>[2x]MAKLTSAVPVLTARDVAEAVEFWTDRLGFSRV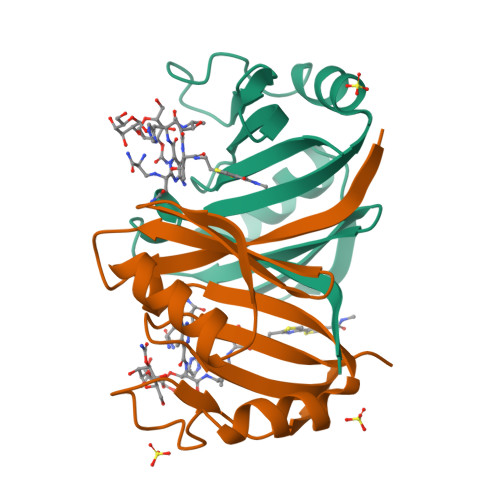FVEDDFAGVVRDDVTLFISAVQDQVVPDNTQAWVWVRGLDELYAEWSEVVSTNFRDASGPAMTEIVEQPWGREFALRDPAGNCVHFVAEEQD2-{2-[(3-carbamoylphenyl)carbamoyl]-6-methoxypyridin-3-yl}-5-{[(2S)-1-hydroxy-3,3-dimethylbutan-2-yl]carbamoyl}benzoic acid | C28 H30 N4 O7 | 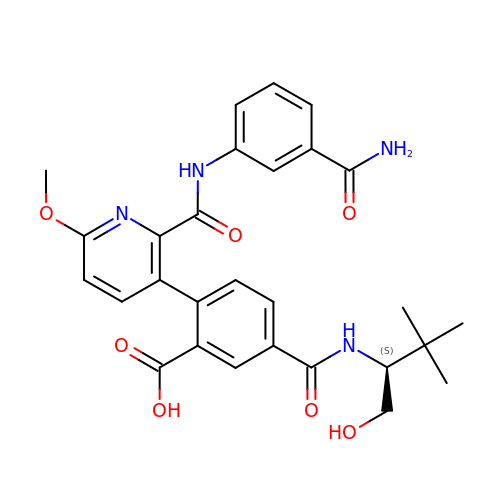QOJVSMMGUMUYEI-OAQYLSRUSA-N> MSDSSEATVKRPLDAHVGPSENAAKKLKIEQRTQADGIHEADVGITLFLSPELPGFRGQIKQRYTDFLVNEIDQEGKVIHLTDKGFKMPKKPQRSKEEVNAEKESEAARRQEFNVDPELRNQLVEIFGEEDVLKIESVYRTANKMETAKNFEDKSVRTKIHQLLREAFKNELESVTTDTNTFKIARSNRNSRTNKQEKINQTRDANGVENWGYGPSKDFIHFTLHKENKDTMEAVNVITKLLRVPSRVIRYAGTKDRRAVTCQRVSISKIGLDRLNALNRTLKGMIIGNYNFSDASLNLGDLKGNEFVVVIRDVTTGNSEVSLEEIVSNGCKSLSENGFINYFGMQRFGTFSISTHTIGRELLLSNWKKAAELILSDQDNVLPKSKEARKIWAETKDAALALKQMPRQCLAENALLYSLSNQRKEEDGTYSENAYYTAIMKIPRNLRTMYVHAYQSYVWNSIASKRIELHGLKLVVGDLVIDTSEKSPLISGIDDEDFDEDVREAQFIRAKAVTQEDIDSVKYTMEDVVL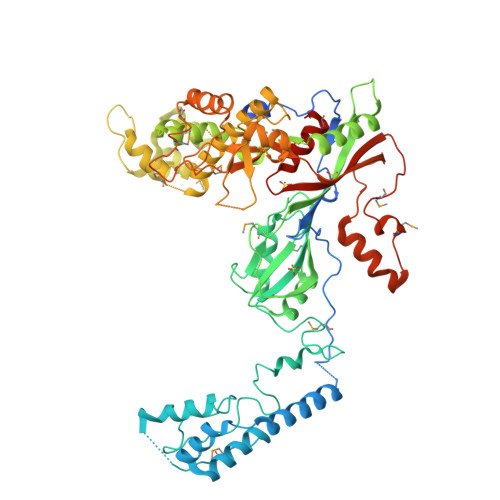PSPGFDVLYPSNEELKQLYVDILKADNMDPFNMRRKVRDFSLAGSYRTVIQKPKSLEYRIIHYDDPSQQLVNTDLDILNNTRAKESGQKYMKAKLDRYMPDKGGEKTAVVLKFQLGTSAYATMALRELMKLETSRRGDMCDVKENI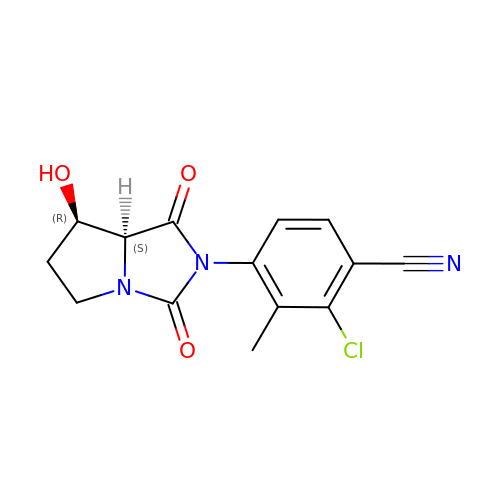2-CHLORO-4-[(7R,7AS)-7-HYDROXY-1,3-DIOXOTETRAHYDRO-1H-PYRROLO[1,2-C]IMIDAZOL-2(3H)-YL]-3-METHYLBENZONITRILE | C14 H12 Cl N3 O3 | KEJORAMIZFOODM-PWSUYJOCSA-N> MKRTALLGLVGAALLGAVPAATVAFAQDAKPELANKLDPNAKEIDEPVLKAATAAKEEDGKYFDKDGHPTFHITNDGKKVDWFTYSGYRRYHAECHVCHGPDGMGSTYAPALKDSLKRLSYEEFYGILAGGKQEISNTANQVMPAFGDNKNVMCYANDLYVYLRARAAGAWGRARPGEKEDKPESA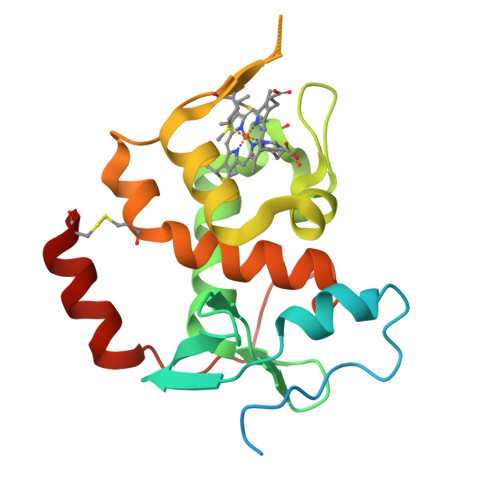KTVEKECLGG>[3x]MKVNNTIVVSIGQAGNQIAASFWKTVCLEHGIDPLTGQTAPGVAPRGNWSSFFSKLGESSSGSYVPRAIMVDLE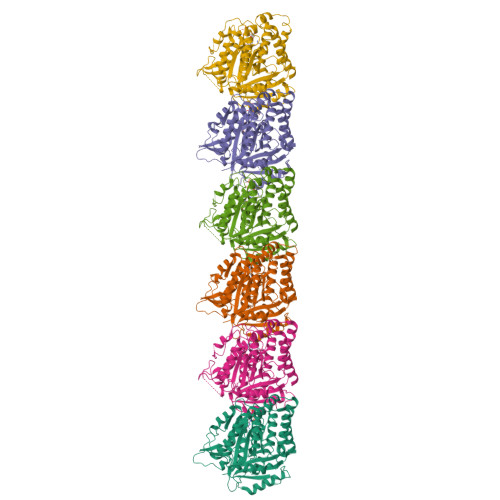PSVIDNVKATSGSLFNPANLISRTEGAGGNFAVGYLGAGREVLPEVMSRLDYEIDKCDNVGGIIVLHAIGGGTGSGFGALLIESLKEKYGEIPVLSCAVLPSPQVSSVVTEPYNTVFALNTLRRSADACLIFDNEALFDLAHRKWNIESPTVDDLNLLITEALAGITASMRFSGFLTVEISLRELLTNLVPQPSLHFLMCAFAPLTPPDGSDGEELGIEEMIKSLFDNGSVFAACSPMEGRFLSTAVLYRGIMEDKPLADAALAAMREKLPLTYWIPTAFKIGYVEQPGISHRKSMVLLANNTEIARVLDRICHNFDKLWQRKAFANWYLNEGMSEEQINVLRASAQELVQSYQVAEESGAKAKVQDSAGDTGMRAAAAGVSDDARGSMSLRDLVDRRR;>[3x]MREILSIHVGQCGNQIADSFWRLALREHGLTEAGTLKEGSNAAANSNMEVFFHKVRDGKYVPRAVLVDLEPGVIARIEGGDMSQLFDESSIVRKIPGAANNWARGYNVEGEKVIDQIMNVIDSAVEKTKGLQGFLMTHSIGGGSGSGLGSLILERLRQAYPKKRIFTFSVVPSPLISDSAVEPYNAILTLQRILDNADGAVLLDNEALFRIAKAKLNRSPNYMDLNNIIALIVSSVTASLRFPGKLNTDLSEFVTNLVPFPGNHFLTASFAPMRGAGQEGQVRTNFPDLARETFAQDNFTAAIDWQQGVYLAASALFRGDVKAKDVDENMATIRKSLNYASYMPASGGLKLGYAETAPEGFASSGLALVNHTGIAAVFERLIAQFDIMFDNHAYTHWYENAGVSRDMMAKARNQIATLAQSYRDAS> MQSGTVQKLLPSAEMLSALLPGLFVAQTRSKTYTSNVMDETRTKRIIDHFAYHKARKQYRASLHNLYSSWRAELVAKQLADPGAQRRLKAEEAREE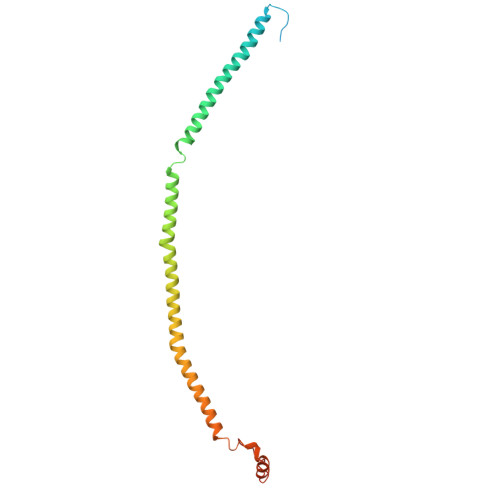AARMAELLREKRVATLVEQVRKAELEHKLAQVQLQRAVRRQEELHRREEARAARYQRLLEASRNWIRQEDLEAAINRALDNPEPFGFVTSLKINRGF> EVTVPDALKDRIALKKTARQLNIVYFLGSDTEPVPDYERRLSELLLYLQQFYGKEMQRHGYGARSFGLDIKSPGRVNIIEYKAKNPAAHYPYENGGGWKAAQELDEFFKAHPDRKKSQHTLIIMPT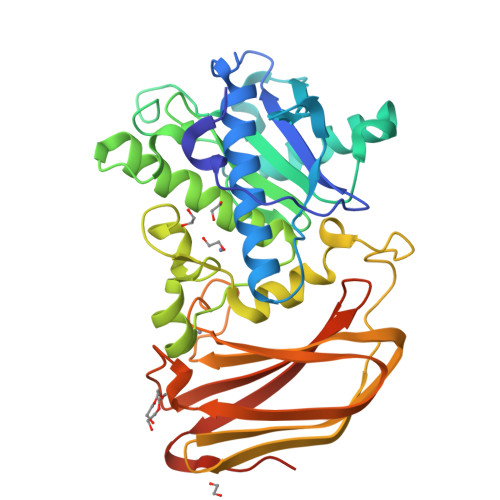WNDEKNGPDNPGGVPFYGMGRNCFALDYPAFDIKHLGQKTREGRLLTKWYGGMAHELGHGLNLPHNHQTASDGKKYGTALMGSGNYTFGTSPTFLTPASCALLDACEVFSVTPSQQFYEGKPEVEVGDVAISFKGDQILVSGNYKSPQTVKALNVYIQDPPYAVNQDYDAVSFSRRLGKKSGKFSMKIDKKELEGLNNNEFRISLMFILANGLHMQKHFTFHWDALQDYRDGSKSGSGHHHHHH>MLGGVRDVLGTLSAVWESGGTAGVGTVVRTFRSAPRPAGASMVVAPDGTVSGSVSGGCVEGAVYDLATEVVATGTPVLQRYGVSDDDAFEVGLTCGGILDVFVEPVSQKTFPQLGAIRDDIEAQRPVAVATVITHPDAQWIGRRLVVHTDEVAGSLGSSRADAAVTDDARGLLAAGRSEVLTYGPDGQRRGEGMEVFVSSYAPRPRMLVFGAIDFAAAVAQQGAFLGYRVTVCDARPVFATTARFPTADEVVVDWPHRYLAAQAEAGAIDARTVVCVLTHDPKFDVPLLEVALRLPDIAYIGAMGSRRTHEDRLARLREAG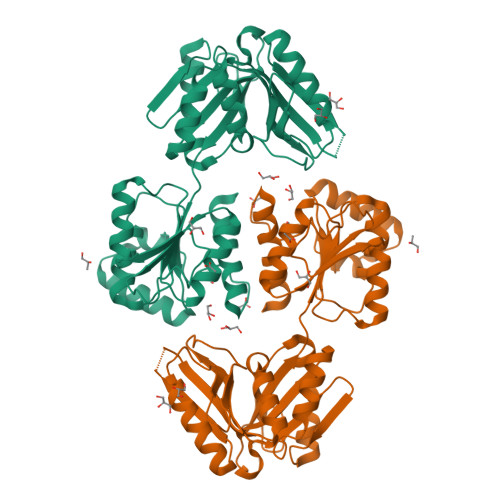LTEEELARLSSPIGLDLGGRTPEETAVSIAAEIIAKRWGGEGRPLAETGGRIHHELGEHESAPAS[2x]>[2x]MRGSHHHHHHGSLLIDKTVIVTGASRGIGRAAARECARQGARVVIGHSGSDEGRAGALSLAEEIAAFGGTAIAVGADAADLDSGEKLVAAAVEAFGSVDVLVNNAGICPFHSFLDMPRELYLKTVGTNLNGAYFTVQAAARRMKEQGRGGAIIAVSSISALVGGAMQTHYTPTKAGLL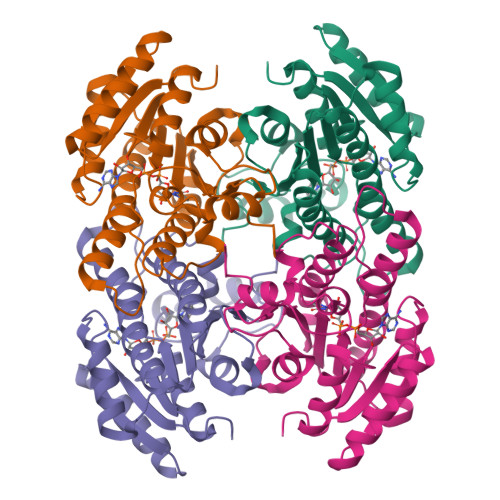SLMQSCAIALGPYGIRCNAVLPGTIATDINKEDLSDLEKRERMTSRVPLGRLGEPDDLAGPIVFLASDMARYVTGASLLVDGGLFVNLQ1,8-dihydroxy-3-methyltetraphene-6,7,12(5H)-trione 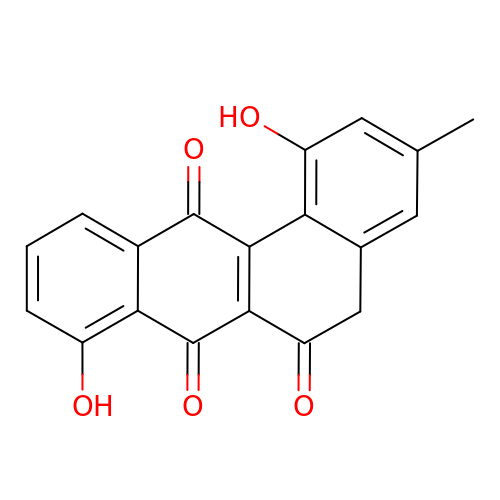| C19 H12 O5 | DFEGERWDHVCALR-UHFFFAOYSA-N> MGSSHHHHHHSQDPENLYFQGTGKFRYMPFSPAGTPFGFTDRRYLTMNEVGYVSTVKNSEQYSITVSFFDVGRFREYHFEDLFGYDLCFLNEKGTLFGQSKTGQIQYRPHDSIHSNWTKIIPLQAGERITSVAATPVR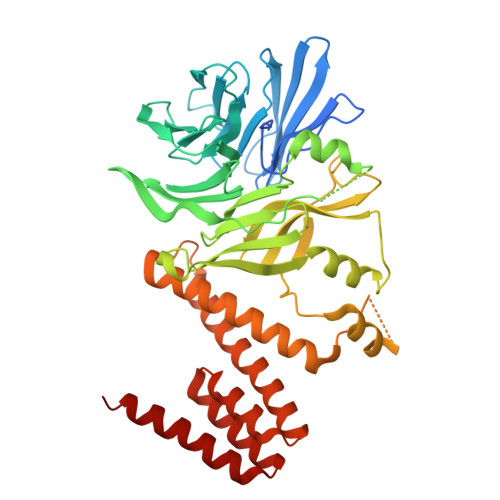VIVGTSLGYFRSFNQFGVPFAVEKTSPIVALTAQNYRVFSVHYSQFHGLSYSLSELGTSSKRYYKRECPLPMSLPNINSDMKKDANLDYYNFNPMGIKSLFFSSYGDPCIFGSDNTLLLLSKWRSPEESKWLPILDSNMEIWKMSGGKETTDIHVWPLALAYDTLNCILVKGKHIWPEFPLPLPSEMEIRMPVFVKSKLLEENKAILNKKNEIGADTEAEEGEEDKEIQIPVSMAAEEEYLRSKVLSELLTDTLENDGEMYGNENEVLAALNGAYDKALLRLFASACSDQNVEKALSLAHELKQDRALTAAVKISERAELPSLVKKINNIREARYEQQLK(1S)-1,5-anhydro-1-(4-bromo-2,5-dihydroxyphenyl)-D-glucitol 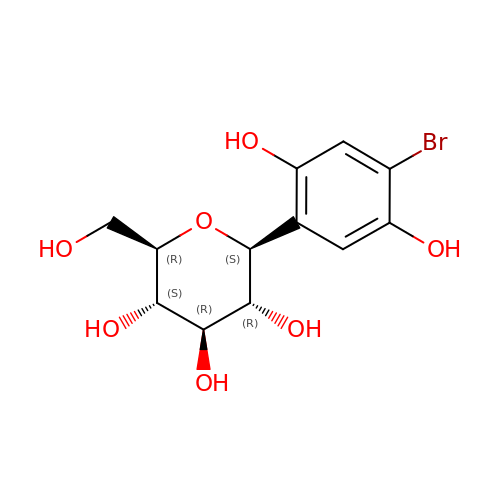| C12 H15 Br O7 | UXXJNKKJRCGMAK-ZIQFBCGOSA-N>[2x]MIPARFAGVLLALALILPGTLCAEGTRGRSSTARCSLFGSDFVNTFDGSMYSFAGYCSYLLAGGCQKRSFSIIGDFQNGKRVSLSVYLGEFFDIHLFVNGTVTQGDQRVSMPYASKGLYLETEAGYYKLSGEAYGFVARIDGSGNFQVLLSDRYFNKTCGLCGNFNIFAEDDFMTQEGTLTSDPYDFANSWALSSGEQWCERASPPSSSCNISSGEMQKGLWEQCQLLKSTSVFARCHPLVDPEPFVALCEKTLCECAGGLECACPALLEYARTCAQEGMVLYGWTDHSACSPVCPAGMEYRQCVSPCARTCQSLHINEMCQERCVDGCSCPEGQLLDEGLCVESTECPCVHSGKRYPPGTSLSRDCNTCICRNSQWICSNEECPGECLVTGQSHFKSFDNRYFTFSGICQYLLARDCQDHSFSIVIETVQCADDRDAVCTRSVTVRLPGLHNSLVKLKHGAGVAMDGQDVQLPLLKGDLRIQHTVTASVRLSYGEDLQMDWDGRGRLLVKLSPVYAGKTCGLCGNYNGNQGDDFLTPSGLAEPRVEDFGNAWKLHGDCQDLQKQHSDPCALNPRMTRFSEEACAVLTSPTFEACHRAVSPLPYLRNCRYDVCSCSDGRECLCGALASYAAACAGRGVRVAWREPGRCELNCPKGQVYLQCGTPCNLTCRSLSYPDEECNEACLEGCFCPPGLYMDERGDCVPKAQCPCYYDGEIFQPEDIFSDHHTMCYCEDGFMHCTMSGVPGSLLPDAVLSSPLSHRSKRSLSCRPPMVKLVCPADNLRAEGLECTKTCQNYDLECMSMGCVSGCLCPPGMVRHENRCVALERCPCFHQGKEYAPGETVKIGCNTCVCRDRKWNCTDHVCDATCSTIGMAHYLTFDGLKYLFPGECQYVLVQDYCGSNPGTFRILVGNKGCSHPSVKCKKRVTILVEGGEIELFDGEVNVKRPMKDETHFEVVESGRYIILLLGKALSVVWDRHLSISVVLKQTYQEKVCGLCGNFDGIQNNDLTSSNLQVEEDPVDFGNSWKVSSQCADTRKVPLDSSPATCHNNIMKQTMVDSSCRILTSDVFQDCNKLVDPEPYLDVCIYDTCSCESIGDCACFCDTIAAYAHVCAQHGKVVTWRTATLCPQSCEERNLRENGYECEWRYNSCAPACQVTCQHPEPLACPVQCVEGCHAHCPPGKILDELLQTCVDPEDCPVCEVAGRRFASGKKVTLNPSDPEHCQICHCDVVNLTCEACQEPGHHHHHH

One extracellular protein family that arose through domain replication and gene duplication is the gel-forming mucins, huge glycoproteins that coat and protect the epithelia in the lungs, intestines, and other organs. A remarkable variation on the theme of mucins arose with the evolution of the complex vasculature in the vertebrate lineage. von Willebrand factor (VWF), a glycoprotein responsible for hemostasis, has a similar domain organization and is homologous to mucins in its amino- and carboxyl-terminal regions. Under acidic conditions, the amino termini of mucins and VWF form noncovalent intermolecular interactions that juxtapose VWD3 assemblies from different CTCK-linked dimers. We present residue-resolution structures of VWF and MUC2 amino-terminal segment tubules, enabling comparison between them and an analysis of the features that stabilize each one.

To compare the two tubules in more detail, we produced tubules of the VWF amino-terminal segment according to a reported method. Due to furin cleavage during recombinant protein production, we assembled the VWF tubules from the D3 dimer and D1D2 fragments purified separately. The VWF and MUC2 tubules also both display twofold symmetry perpendicular to the helix axis. They differ, however, in that the VWF tubule is a one-start helix, whereas the MUC2 tubule is a two-start helix. The VWF tubule has a helical twist of 86.0° (about 4.2 subunits per turn) and an axial rise of 2.85 nm per subunit. These values are in close agreement with previous results, which reported a helical twist of 85.6° and an axial rise of 2.62 nm for the low-resolution reconstruction of the VWF tubular scaffold. Density maps showed that the region around the furin cleavage site was exposed and flexible. The region surrounding the furin cleavage site was disordered and could not be modeled, but its junctions with the rest of the protein clearly indicate that the cleavage site is exposed in the “window” of the VWF tubule, which has dimensions of about 7 × 6 nm. Thus, the structure of the VWF tubule is consistent with furin cleavage occurring after tubule assembly in vivo. The MUC2 tubule thus appears to be stabilized mainly by quaternary interactions between turns of the helix, whereas the more rigid packing of the bridge in VWF appears to dictate the geometry of its tubule. The residue-resolution structure of VWF, presented here, enabled an analysis of the molecular features that produce the tight, one-start helix previously visualized only at low resolution or by homology modeling.> MESGIDLQGQFISALQSLGLSHDLAKLLWLPLPMLMMLIVATVGVLVAVWLERKISAAVQQRIGPEYIGPLGILAPLADGLKLIFKEDVLPANSDRWLFTLGPAVVVIPVFLSYIIVPFGQNLLISNLAMGVFLWIALSSIAPIGLLMAGYASNNKYSLLGGLRAAAQSISYEIPLALAVLAVAMMSNGLGTVEIVEQQSQYGILSWNVWRQPIGFLVFWIAALAECERLPFDLPEAEEELVAGYQTEYAGMKFALFYLGAYVNLVLSALLVSVLYFGGWSFPIPLETIANLLGVSETNPFLQIAFAVLGITMTLIKAYFFVFLAILLRWTVPRVRIDQLLDLGWKFLLPVGLVNLLLTAGLKLAFPVAFGG;> MDLVTLAGQLNAGTILPETILIVTLLVVLLADLIQGRQADRWTPYFAIVGLGGAIATMIPLWTQPATISFFGSFISDHLSLFFRGLIALSALGTILMSIRYVEQTGSSLGEFMTILLTATVGGMFIAGAQELVFIFVALETLSIASYLLTGYTKRDSRSNEAALKYLLIGAASSAIFLYGSSLLYGLSGGHTQLPAIAQALSSESLGLVVALVFVIAGISFKISAVPFHQWTPDVYEGAPTPVVAFLSVGSKAAGFALAIRFLTLAFPSVTDQWQLIFTVLAILSMILGNVVALAQTSMKRMLAYSSIGQAGFVMIGFVVGTEAGYASMLFYLLVYLFMNLGAFTCVILFSLRTGTDQISEYAGLYQKDPLLTLGLSLCLLSLGGIPPLAGFFGKIYLFWAGWQAGAYGLVLLGLLTSVISIYYYIRVVKMMVVKEPQEMSEAVRNYPEVSWSSFGLRPLQVGLVMTVIATSLAGILANPLFNLVNTAVWDVPQLANQPTVMEVAYQALSPAGKS;> MVAIPRLRDTATVFVLSGYEYFLGFLIICSLVPVLALAASALLRPKSGRMIRLTTYESGMEPIGGAWIQFNVRYYMFALVFVIFDVETVFLYPWAVAFHQLGLLAFIEALIFIAILVVALVYAWRKRALEWS;> MSTFPWLTTIILFPIVAALAIPFIPDPTGKGRPIRWYALAVGLIDFALIVYAFTNFYDLNTPGMQLWESYDWIPEIGLRWSVGADGLSMPLILLTGFITTLAILAAWPVTLKPRLFYFLMLAMYGGQIAVFAVQDMLVFFLAWELELIPVYLLLAIWGGHKRQYAATKFILYTAGSSLFILVAGLAMAFYGDTVSFDMQTLAAKDYALGFQLLVYAGFLVAYGVKLPIVPLHTWLPDAHGEATAPVHMLLAGILLKMGGYALIRMNVDMLPAAHAKFAPVLVILGVVNIIYAALTSYAQRNLKRKIAYSSISHIGFVLIGIASFTNLGMSGAVLQMVSHGLIGASLFFLVGATYDRTHTLILEEMGGVGQKMKKIFAMFTACSLASLALPGMSGFVAELMVFIGFATSDAYSLPFRVIVVFLAAVGVILTPIYLLSMLREIFYGPENKELVEHEALVDAEPREVFIIACLLVPIIGIGLYPKLLTQIYDATTGQVIARAREVLPTLAQQTEQPLGILPMVAPQLKANAQ;> MQLTYVLILAALLFCIGIYGLVTSRNAVRVLMSIELLLNAVNLNLIGFANYLDGQQIKGQVFAVFVITVAAAEAAVGLAIILAIYRNRDTVDMEKFNLLKW;> MEPLYQYAWLIPVLPLLGALIVGFGLIAFSETTSKLRRPSAIFIMALMAIAMGHSLTLFWSQVQGHLPYTQMIEWAAAGNLHIAMGYVIDPLAALMLVIVTTVAFLVMLYSDGYMAHDPGYVRFFAYLSLFGSSMLGLVVSPNLVQVYIFWELVGMCSYLLIGFWYDRKSAAEAAQKAFVTNRVGDFGLLLGMVGLFWATGTFDFAGMGDRLTELVNTGLLSPSLAAILAILVFLGPVAKSAQFPLHVWLPDAMEGPTPISALIHAATMVAAGVFLIARMFPVFEQLPQVMTTIAWTGAFTAFMGATIAITQNDIKKSLAYSTISQLGYMVMGMGVGAYSAGLFHLMTHAYFKAMLFLGSGSVIHSMEGVVGHNPDLAQDMRYMGGLRKYMPITGATFLVGCLAISGVPPFAGFWSKDEILGAVFHANPAMWLLTWLTAGLTAFYMFRMYFMTFEGKFRNVPPERQEHHDHHSHHAAVPHESPWTMTLPLVVLAIPSTLIGFVGTPFNNLFEVFIHAPGEEKVAEHAVDLTEFLILGGSSVGIGLMGITVAYLMYLKGTPSPQAIAKAIQPLYQFSLHKWYFDELYEAVFIKGCRRLARQVLEVDYNVVDGVVNLTGFVTMVTGEGLKYLQNGRAQFYALIVLLAVLGFVIFSVQT;> MDLATLTQTITFFALAAAVIIAALGVVLLDNVVYSAFLLGGVFLSIAGLYILMNADFVSAAQILIYVGAVNVLILFAIMLVNKRETYTPVPGRWLRQGGAAVVSLGVFALLTKMILQTPWQLSSVPPTPDSITTIGQHFFSDFLLPFELASVLLLMALIGAVVLARRELVLEPEPILGEEVVPPLELPERPREPVALSEK;> MPKIETRTEPMVINMGPHHPSMHGVLRLMVTLDGEDVIDCEPVIGYLHRGMEKIAENRTNIMFIPYVSRWDYAAGMFNEAVTVNAPEKLAGIPVPKRASYIRVIMLELNRIANHLLWLGPFLADVGAQTPFFYIFREREYIYDLFEAATGMRFINNNYFRIGGVAADLTYGWVTKCRDFCDYFLPKVDEYERLITNNPIFVRRLQGVGKISREEAINWGLSGPMLRASGVKWDLRKVDHYECYDDFDWDVPVATEGDCLARYIVRIQEMRESVKIIRQALDGLPGGPYENLEAKRMLEGAKSEWNGFDYQYIGKKLSPTFKIPKGEHYVRVESGKGELGIYLIGDDNVFPWRWKIRPPDFNNLQVLPQLLKGMKVADIVAILGSIDVIMGSVDR;> MKFLNQITNYAKEAVQSAKYIGQGLSVTFDHMRRRPITVQYPYEKLIPSERFRGRIHFEFDKCIACEVCVRVCPINLPVVDWVFNKELKKKELKHYSIDFGVCIFCANCVEYCPTNCLSVTEEYELATYDRHELNYDSVAMGRIPYKVTQDPMVTPIREFAYLPAGVMSGHDLPAGAQRAGERPEAIANTAKSSEN;> MSDTPEAPIVEAGPVGRLLQSQNLSVESLGRDASGVEMIKVDRDRLLAVCQTLYADGFNYLRCQAAYDSGPGQDLVSTYHLIKLSDNADRPPEVRIKVFVPRDDPRVPSVYWIWKTADWQERESYDMFGIVYEGHPNLKRILMPEDWVGWPLRKDYITPDFYELQEAY;> MTNTTSPAILNPIARPEVPQELAENIILTSLNDVYDWARLSSLWPLMYGTACCFIEFAAMIGSRFDFDRFGLVPRNSPRQADLIITSGTITMKMAPALVRLYEQMPSPKYVIAMGACTITGGMFSSDSYSAVRGVDKLIPVDVYLPGCPPRPEAIMDAIVKLRKKIANEHINERGNLAQTHRLFTAKHKMKPVPPILTGQYLNAPSRQAPPPALAAAMGIAVPALGEAVSETTSVAE;> MAVSTELLVLGVYGALAGLYLLVVPAIVYAYLNARWYVASSFERAFMYFLVTFFFPGLLLLAPFINFRPQPRSLNS;> MLLKSTTRHVHIYAGHVVDGEVHPDT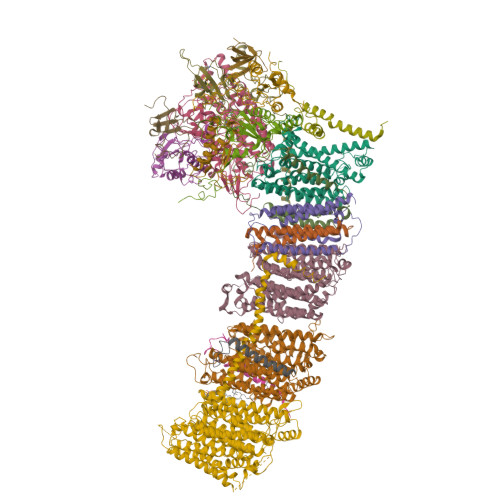ETLTLNVDPDNELEWNEAALAKVEAKFRELVANAAGEDLTEYNLRRIGSDLEHFIRSLLMQGEIGYNLNSRVRNYSLGIPRVNHS;> MGLLAGYQFVKDLESAGALALFVPPEGGFEGRYQRRLRSKGYTTLPMSAPGLGDLAAYLTQEHGIRPAHTGKEDIRVYFQPPLVTYHLENLPPNAKGLVLWLIDGKRLSKQEFAYLAQLTQTLPKFKVVVEVGGDRVVRWEPLADWVAAA;> MAIKKGDLVKVVAEKLANSLEALASDHRYPPYLFEGRGEVVDIRGDYAQIKFPVPTPTVWLRLDQLEVAQ;> AVISVKPILLAMTPVFILLCLFFGTRNGFYDTDQYHGNAAAH;> ATDFRAIMKFDGADSPAMIAISAVLILGFIAGLIWWALH;> MIRPIADTYPLLPLSKAQMGQRQEIINSHKRLWDKTMATDLIMTILPGMTVKVTNPNDTYYQFQGIVQRITDGKVAVLFEGGNWDKLVTFQASELEPVVVTPKEKAKAKK>MGVNANISESLTGTIEAPFPEFEAPPANPMEVLRNWLERARRYGVREPRALALATVDGQGRPSTRIVVIAELGERGVVFATHADSQKGRELAQNPWASGVLYWRESSQQIILNGRAERLPDERADAQWLSRPYQTHPMSIASRQSETLADIHALRAEARRLAETDGPLPRPPGYCLFELCLESVEFWGNGTERL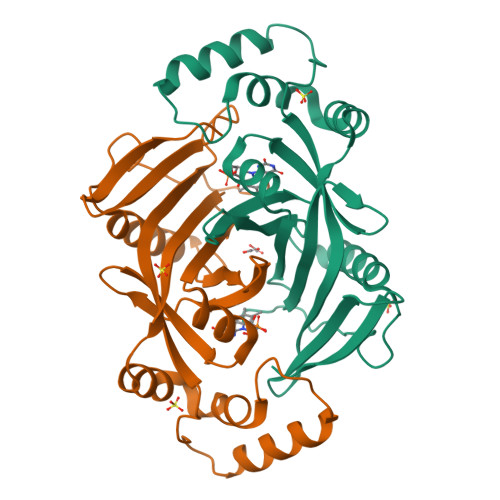HERLRYDRDEGGWKHRYLQP[2x]Nitrocefin - open form | C21 H18 N4 O9 S2 | 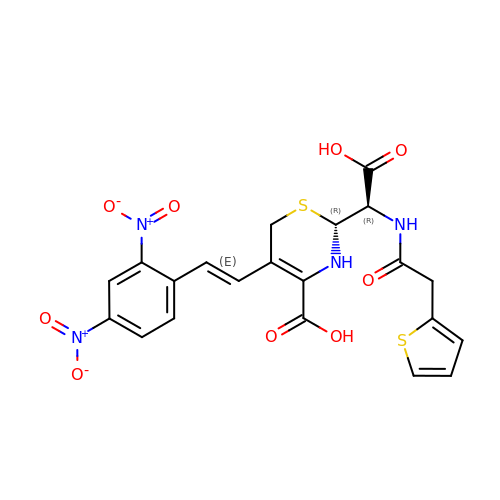PYBZXZZHQKFSGC-CZHQAMEJSA-N>[5x]SNAMIIRPEQHWFLRLFDWHGSVLSKIIFRLLLNVLMSIIAIISYQWYEQLGIHLTVAPFSLLGIAIAIFLGFRNSASYSRFVEARNLWGTVLIAERTLVRQLRNILPAEHDAHRRIVSYLVAFSWSLKHQLRKTDPTADLRRLLPEERVTEILASSMPTNRILLLAGNEIGQLREAGKLSDITYGLMDNKLDELAHVLGGCERLATTPVPFAYTLILQRTVYLFCTLLPFALVGDLHYMTPFVSVFISYTFLSWDSLAEELEDAFGTAANDLPLNAMCNTIERNLLDMTGQHPLPE

Human bestrophin1 (hBest1) is a Ca2+-activated Cl− channel essential for Cl− transport in retinal pigment epithelium (RPE). Although the structure of hBest1 is still unsolved, two Best1 homolog structures, one from bacteria Klebsiella pneumoniae (KpBest) and the other from chicken (cBest1), have been previously reported. Overall, the channel is a pentameric assembly with a single ion-conducting pathway, which varies in diameter along its length and is constrained at two narrow points: a “neck” contributed by three residues (I62/I66/F70 in KpBest and I76/F80/F84 in hBest1/cBest1) on a transmembrane helix, and an “aperture” formed by a single residue (I180 in KpBest1, I205 in hBest1, and V205 in cBest1) on a cytosolic helix. Here, by electrophysiological and structural analyses, we show that the neck and aperture in hBest1 are both indispensable Ca2+-dependent gates, and their dysregulated opening by rationally designed or patient-derived mutations causes Ca2+-independent leak and elevates Ca2+-dependent channel activity.

Alanine substitution mutants for each of the 12 residues were generated in KpBest and hBest1 and subjected to crystallography and patch clamp, respectively. Moreover, the equivalent KpBest mutants (W16A, G18A, S19A, L259A, P262A, G264A, and D269A) all showed an overall similar structure to that of WT KpBest. The corresponding “Ca2+-binding” sites in WT KpBest are occupied by Zn2+, an essential component in the crystallization buffer. Interestingly, the KpBest P262A, G264A, and D269A mutants show no Zn2+ in the corresponding sites. Moreover, KpBest L259A, P262A, G264A, and D269A all have relatively low resolution and slightly altered structures in this region, suggesting that the binding of Zn2+ stabilizes the channel structure.DEOXYCYTIDINE DIPHOSPHATE | C9 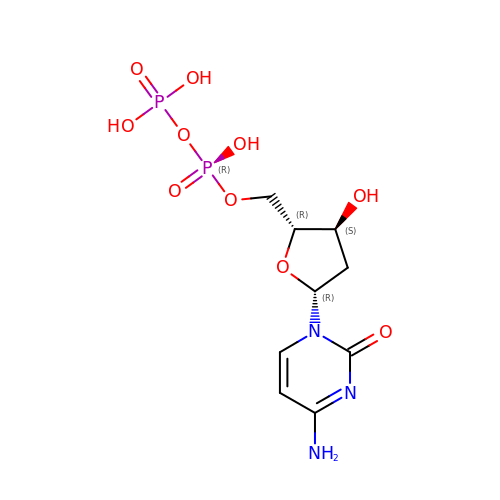H15 N3 O10 P2 | FTDHDKPUHBLBTL-SHYZEUOFSA-N4-(trifluoromethyl)-1,5,6,7-tetrahydro-2H-cyclopenta[b]pyridin-2-one | C9 H8 F3 N O | 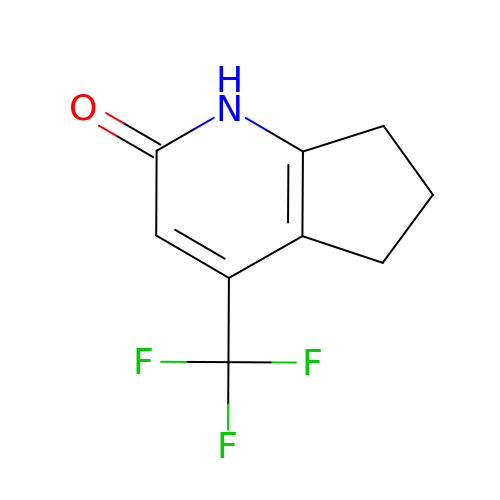GSJGKNLMGQIWJH-UHFFFAOYSA-N>GSHMAVQIGFLLFPEVQQLDLTGPHDVLASLPDVQVHLIWKEPGPVVASSGLVLQATTSFADCPPLDVICIPGGTGVGALMEDPQALAFIRQQAARARYVTSVATGSLVLGAAGLLQGKRATTHWAYHELLAPLGAIPVHERVVRDGNLLTGGGITAGIDFALTLAAELFDAATAQRV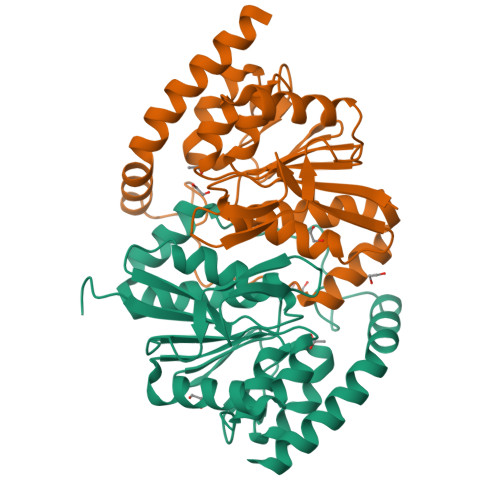QLQLEYAPAPPFNAGSPDTAPASVVQQARQRAADSLHKRREITLRAAARLAAG[2x]> DNPGTAPLDTFMTLSESLTGKKGLSRVIGERLLQALQKGSFKTADSLPQLAGALASGSLTP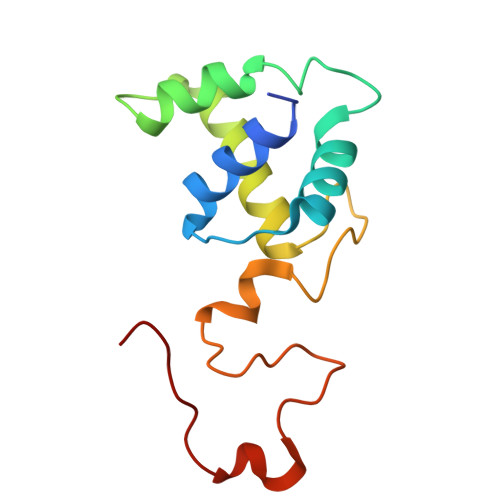EQESLALTILEAWYLGIVDNVVITYEEALMFGVVSDTLVIRSYCPNKPGFWADKPIERQA>[2x]MELKNSISDYTEAEFVQLLKEIEKENVAATDDVLDVLLEHFVK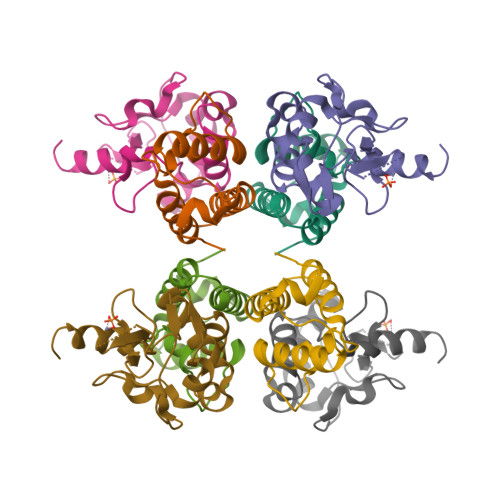ITEHPDGTDLIYYPSDNRDDSPEGIVKEIKEWRAANGKPGFKQG;>KRNKPGKATGKGKPVNNKWLNNAGKDLGSPVPDRIANKLRDKEFKSFDDFRKKFWEEVSKDPELSKQFSRNNNDRMKVGKAPKTRTQDVSGKRTSFELHHEKPISQNGGVYDMDDISVVTPKRHIDIHRGK[2x]>DTSSLIVEDAPDHVRPYVIRHYSHARAVTVDTQLYRFYVTGPSSGYAFTLMGTNAPHSDALGVLPHIHQKHYENFYCNKGSFQLWAQSGNETQQTRVLSSGDYGSVPRNVTHTFQIQDPDTEMTGVIVPGGFEDLFYYLGTNATDTTHTPYIPSSSDSSSTTGPDSSTISTLQSFDVYAELSFTPRTDTVNGTAPANTVWHTGANALASTAGDPYFIANGWGPKYLNSQYGYQIVAPFVTATQAQDTNYTLSTISMSTTPSTVTVPTWSFPGACAFQVQEGRVVVQIGDYAATELGSGDVAFIPGGVEFK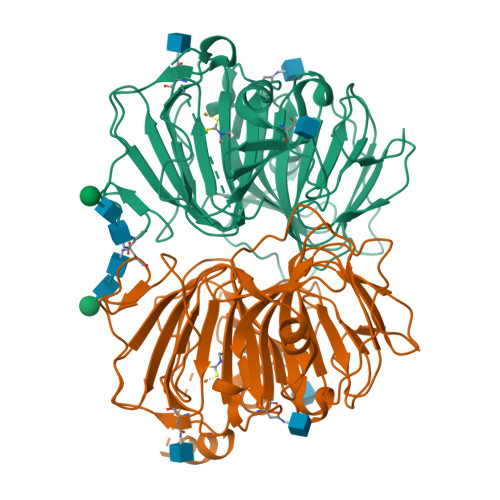YYSEAYFSKVLFVSSGSDGLDQNLVNGGEEWSSVSFPADW[4x]N-[(1S,2R,3R,4S,5R)-3,4,5-trihydroxy-2-methylcyclohexyl]acetamide | C9 H17 N 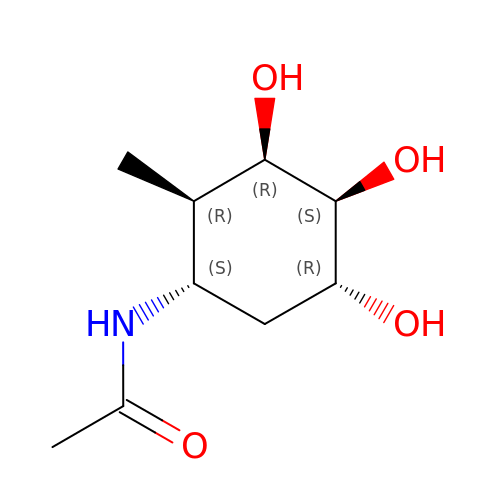O4 | KFWZFLHIHNMMRU-ACWCSBLCSA-N> MLTRQARLLRRIPPPNAVLQSGLQRRHRSTDRYSNNIHTSSTQNAPAPVYDTPIREKGMTLEAKERVRAHVRKIQSSASTAAASPAVRPQPAQHFQAAPQPMPTNMPRFESDSQVKNGLDYSFIGLSGGQIFQEMMLRHDVKQVFGYPGGAILPVFDAIYNSPHFEFVLPRHEQGAGHMAEGYARVSGKPGVVLVTSGPGATNVITPMQDALSDGVPMVVFCGQVATNLIGSDAFQEADVVGISRSCTKWNVMVKDIAELPRRINEAFKIATTGRPGPVLVDLPKDVTAAILRTPIPAKSVQPGHSPYLPSNPLNPSSQPSDPLPGDADLITEAAQMINKAKRPIIFAGNGVLSSPEGPKLLKELSDKGRIPVTTTLQGLGAFDERDEKSLHMIGMHGSAYANFAMQEADVLIALGVRFDDRVTGKVDTFAPAAKAAAAEGRGG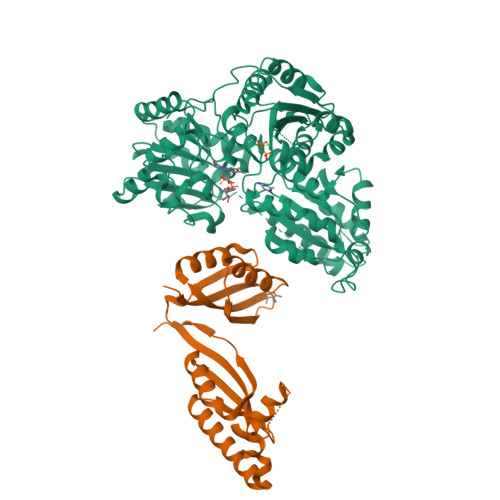IIHFEIQPKNINKIVEGQIPVLGDVVASLGELVPQIEAVDRSAWIGRCKATKERYPFTYTPSQEGQKLKPQEVVQELDRQAEALGKEKFVISTGVGQHQMWACQYYRWTEPRSWVSSGGLGTMGFGLPSAIGAKVAAPEKYVIDIDGDASFSMTAMELATASQYDIGVKVLLFNNEFQGMVEQWQDLFYENRYSRTRMTNPDFVKLSESMGAKGLRCTKLEDLPRMMKEFLEYDGKRPIVLECLVSSEHVYPMIPAGKALHEQLLHPLLRNGSE;> MLRSLLQSGHRRVVASSCATMVRCSSSSTSALAYKQMHRHATRPPLPTLDTPSWNANSAVSSIIYETPAPSRQPRKQHVLNCLVQNEPGVLSRVSGTLAARGFNIDSLVVCNTEVKDLSRMTIVLQGQDGVIEQARRQIEDLVPVYAVLDYTNSEIIKRELVMARISLLGTEYFEDLLLHHHTSTNAGAADSQELVAEIREKQFHPANLPASEVLRLKHEHLNDITNLTNNFGGRVVDISETSCIVELSAKPTRISAFLKLVEPFGVLECARSGMMALPRTPLKTSTEEAADEDEKISEIVDISQLPPG> MHHHHHHGSGMALAIKKRVGTYVETVDGSPPVKKLRLQTLAADAKGGKSGKVGNVERKLTALNQLDAYVGNLPAGALVLPTGTPVASTGAPSTGVIGNPPAAATGAPPMTAANSRELLELLVKITDEISYEDVEMGELKEVASKIFQLYQLQERDSDTSIRVKLLELLSGLGCECATEQALTMIIDYFIFLLRKEVSQKVLAQGMMCLFRIGERRKHMLPISYKTQVAHLAKEQLRSGSAHTQKNAMLVIGRFATKMEGERHYVWKLAFYIDSQDSSVRAQALHALLTLGERGSQLPAVLYKRAVEAMKDDYECVRKEALQLVFMLGNRHPDYILPSDRQQEELRMIDAAFSKVCEALCDLSLQIRVLAAELLGGMTAVSREFLHQTLDKKLMSNLRRKRTAHERGARLVASGEWSSGKRWADDAPQEHLDAQSISIIASGACGALIHGLEDEFLEVRTAAVASMCKLALSRPDFAVTSLDFLVDMFNDEIEDVRLKAIYSLTAIAKHIVLREDQLEIMLGSLEDYSVDVREGLHLMLGACRVSTQTCLLMVVQKLLDVLAKYPQDRNSTYACMRKIGQKHPHLVMAVAVHLLYVHPFFETPERDVEDPAYLCVLILVFNAAEHLVPIISLLPTATHRHYAYLRDSMPNLVPQLPIEGASSASATHRIDSAMHQAGSSAEYLQMILSHIEEIFTMTDERLELLQTAQSNLQRLGSIDAGMYGTSNFLETFLAAQIQIEQMQRCASTQRSRVPLKESLAALIRNCLKLQHTFSGLNYGDILQVKQLRLRACALHLVLVVRDRSQSALGPCQMLLQTAGDISEFIKANTKDEEEKPPVVETDMPMKESVSRDAQPDSFTRQLLIKLDGISDPKPGRVFREILPLVQQAPPLALPPANDKIRRCVANILEPCPLQSQDNVIKVTAGLIAAVPFVAEIDNLLESQKADMRIKIKYPDQHMHTVVPKQSDFKPIMTEQGEHKTNVRLRTTILLSHSVWTESSLVEIQLCLAVRPGSELELCKPAKVLFAPKPVRRGI;> MRLYCLSGDLAKPCYIITFKGLRIMLDCGLTEQTVLNFLPLPFVQSLKWSNLPNFVPSRDHDPQMDGELKDCCGRVFVDSTPEFNLPMDKMLDFSEVDVILISNYLNMLALPYITENTGFKGKVYATEPTLQIGRFFLEELVDYIEVSPKACTARLWKEKLHLLPSPLSEAFRAKKWRTIFSLKDVQGSLSKVTIMGYDEKLDILGAFIATPVSSGYCLGSSNWVLSTAHEKICYVSGSSTLTTHPRPINQSALKHADVLIMTGLTQAPTVNPDTKLGELCMNVALTIRNNGSALIPCYPSGVVYDLFECLTQNLENAGLNNVPMFFISPVADSSLAYSNILAEWLSSAKQNKVYLPDDPFPHAFYLRNNKLKHYNHVFSEGFSKDFRQPCVVFCGHPSLRFGDAVHFIEMWGNNPNNSIIFTEPDFPYLQVLAPFQPLAMKAFYCPIDTSLNYQQANKLIKELKPNVLVIPEAYTKPHPSAPNLFIEQPDKKIITFKCGEIIRLPLKRKLDRIYITSELAQKISPKEVAAGVTFSTLTGVLQVKDKVHCIQPCADSVKDETISSNSAPTKEDVLKNVKYEYGSIDVDAVMKKLAQDGFSNIKLDRTGGALTLNLVNEDTVIKFEDNETHIICGGKPTTRLKLRDTIMKCLQSF;> MPDIKITPLGAGQDVGRSCLLLSMGGKNIMLDCGMHMGYNDERRFPDFSYIVPEGPITSHIDCVIISHFHLDHCGALPYMSEIVGYTGPIYMTHPTKAIAPILLEDMRKVAVERKGESNFFTTQMIKDCMKKVIPVTLHQSMMVDTDLEIKAYYAGHVLGAAMFWIKVGSQSVVYTGDYNMTPDRHLGAAWIDKCRPDLLISESTYATTIRDSKRCRERDFLKKVHECVAKGGKVLIPVFALGRAQELCILLETYWERMNLKYPIYFALGLTEKANTYYKMFITWTNQKIRKTFVHRNMFDFKHIKPFDKAYIDNPGAMVVFATPGMLHAGLSLQIFKKWAPNENNMVIMPGYCVQGTVGNKILGGAKKVEFENRQVVEVKMAVEYMSFSAHADAKGIMQLIQNCEPKNVMLVHGEAGKMKFLRSKIKDEFNLETYMPANGETCVISTPVKIPVDASVSLLKAEARSYNAQPPDPKRRRLIHGVLVMKDNRIMLQNLTDALKEIGINRHVMRFTSKVKMDDSGPVIRTSERLKTLLEEKLAGWTVTMQENGSIAIESVEVKVEEDEKDPKQKNILISWTNQDEDIGAYILNVLQNMC

Integrator is a multi-subunit protein complex associated with RNA polymerase II (Pol II), with critical roles in noncoding RNA 3′-end processing and transcription attenuation of a broad collection of mRNAs. IntS11 is the endonuclease for RNA cleavage, as a part of the IntS4-IntS9-IntS11 Integrator cleavage module (ICM). For example, our earlier studies have shown that IntS4-IntS9-IntS11 forms the Integrator cleavage module (ICM). IntS9 and IntS11 are paralogs of CPSF100 and CPSF73 in the canonical and U7 replication-dependent histone pre-mRNA 3′-end processing machineries, and CPSF73 catalyzes the cleavage reaction in both machineries.

Here we report a cryo-EM structure of the Drosophila ICM at 2.74 Å resolution, which unexpectedly reveals the stable association of an inositol hexakisphosphate (IP6) molecule. The structure shows that the C-terminal segments of IntS9 and IntS11 contain two separate domains, CTD1 and CTD2, similar to their paralogs CPSF100 and CPSF7317. The metallo-β-lactamase and β-CASP domains of IntS9 and IntS11 form a pseudo-dimer in this structure, remarkably similar to the pseudo-dimer for the equivalent domains of CPSF100 and CPSF73 in the active U7 machinery. The N-terminal domain (NTD) of IntS4 contacts the metallo-β-lactamase domain of IntS9 and the back face of IntS11 metallo-β-lactamase and β-CASP domains, which may promote the formation of this pseudo-dimer. The structure of Drosophila ICM unexpectedly revealed the presence of an inositol hexakisphosphate (IP6) molecule, with good quality EM density. IP6 is located at an interface among all three subunits of the ICM, formed by the N-terminus and the linker to CTD1 of IntS9, the CTD1 of IntS11, and the first few helical repeats of IntS4 NTD. IP6 has ionic interactions with all three subunits, including Lys189 of IntS4, the N-terminal ammonium ion, Arg2, Arg504, Lys508 and Arg509 of IntS9, and Lys462 of IntS11. These residues create a large, highly positively charged pocket, accommodating IP6 or other highly negatively charged molecules. The 2-phosphate interacts with Arg504 and Lys508 of IntS9, suggesting that IP5, which lacks this phosphate, would have weaker interactions with ICM. The binding site for IP6 in ICM is located far (55 Å) from the active site of IntS11 and is on the opposite face from the opening for the canyon in IntS11 for binding RNA.> 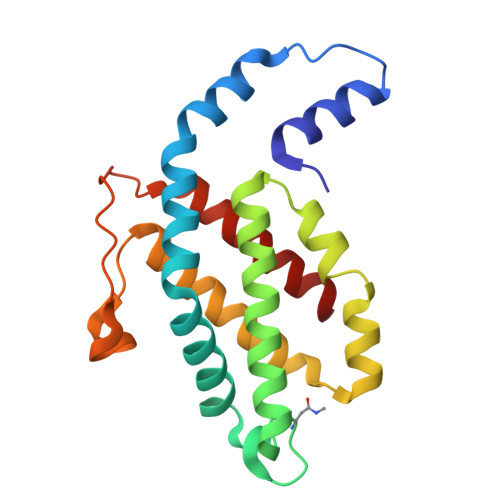MLDAFSRAVVQADASTSVVADMGALKQFIAEGNRRLDAVNAIASNASCMVSDAVAGMICENQGLIQAGGNCYPNRRMAACLRDAEIILRYVTYALLAGDASVLDDRCLNGLKETYAALGVPTTSTVRAVQIMKAQAAAHIKDTPSEARAGGKLRKMGSPVVEDRCASLVAEASSYFDRVISALS>MSNLDELASSRQTVLEPQDEVRIVGQYYDDKTAKLVRKYGPGPRIHYHVGYYPSSEAPRHTRDVTPDAFRRSIRLHQEGLLRYAAKIWGAEHRLSGRILDVGCGLGGGSLFWAQEYGADVTAVTNAPEHAPIVEGFARECGVGGRVRTLVCDAMHLPLDGGPYDAAVAIESS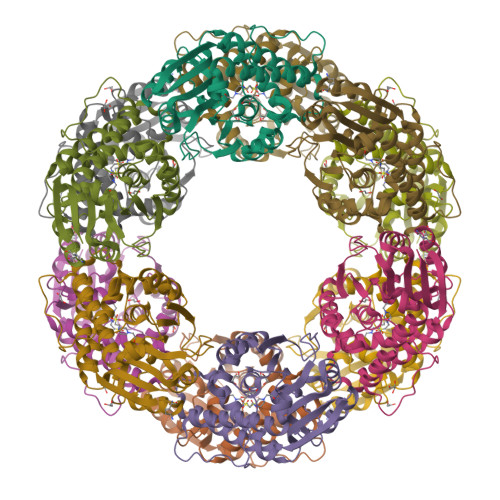GYFDRPVWFERLAHVLRPGGSVCIEEVFTTRPHGADVWAEYFYTKPATVLDYAEAAKAAGFELVDDVDATSETLPFWEESTAWTKAVLDSDSTLSAVDRRQLRISLMANQALGAEWQAGGLRLGFLRFERK[3x]>[6x]MTRRYLKYYIFVTLLFFVQVINNVLCAPDNKQEQGKYLNRTINILNAGKNIAKSYGHNKLKPIHILSALAKSDYGSTLFKENNVNAANLKEYIDIALEQTRAGAPLDNKSKIVNSAEVKETLALAEAAANKYKSPKVDVEHLLSGLSNDELVNEIFNEVYLTDEAIKAILKRKFEKTKKDKDGKTGTLYIEQFGSNMNEKVRNGKLQGIYGRDEEIRAIIESLLRYNKNSPVLVGNPGTGKTTIVEGLVYRIEKGDVPKELQGYTVISLNFRKFTSGTSYRGEFETRMKNIIKELKNKKNKIILFVDEIHLLLGAGKAEGGTDAANLLKPVLSKGEIKLIGATTIAEYRKFIESCSAFERRFEKILVEPPSVDMTVKILRSLKSKYENFYGINITDKALVAAAKISDRFIKDRYLPDKAIDLLNKACSFLQVQLSGKPRIIDVTERDIERLSYEISTLEKDVDKVSKKKYNKLI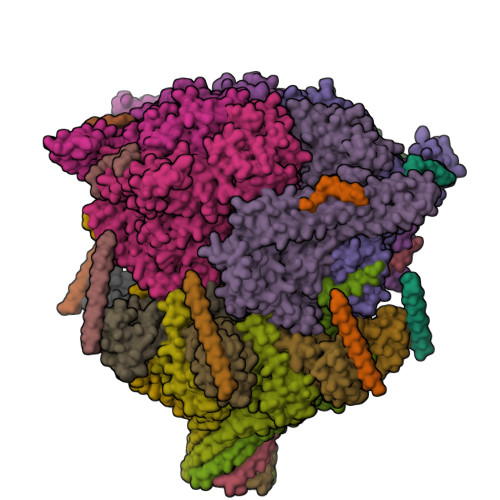KEFEEKKEQLKKYYEEYVITGERLKRKKEIEKKLNDLKELTQNYVYSNKEPPIELQNSLKEAQQKYLELYKETVAYVEAKTHNAMNVDAVYQEHVSYIYLRDSGMPLGSLSFESSKGALKLYNSLSKSIIGNEDIIKSLSDAVVKAATGMKDPEKPIGTFLFLGPTGVGKTELAKTLAIELFNSKDNLIRVNMSEFTEAHSVSKITGSPPGYVGFSDSGQLTEAVREKPHSVVLFDELEKAHADVFKVLLQILGDGYINDNHRRNIDFSNTIIIMTSNLGAELFKKKLFFDADNSGTPEYKRVMEDVRLSLIKKCKKVFKPEFVNRIDKIGVFEPLNKKNLHKIVALRFKKLEKRLEEKNIQVSVSEKAIDYIIDQSYDPELGARPTLIFIESVIMTKFAIMYLKKELVDDMDVFVDYNSKAKNLVINLSKT;>MKVSYIFSFFLLFFVYKNTNTVVCDNGYGDLAATSALTTVIKDPISLTIKDIYEHGVKNPFTKIIHKLKKFIRYRKVLRWSRMWWVLLVREIVGDNTIEKKTEKALREIWDQCTIAVYNNTLNAVESKPLLFLHGILNECRNNFATKLRQDPSLIVAKIDQIIKSQIYRFWVSEPYLKIGRSHTLYTHITPDAVPQLPKECTLKHLSSYMEEKLKSMESKKNIESGKYEFDVDSSETDSTKDDGKPDDDDDDDDNFDDDDNFDDDTVEEEDASGDLFKNEKKDENKE[7x];>MRIIILALLIVCTIINYYCAVQNNGNKSLNVMPTCSMPGNDSDSNDNETGDVDNDKNNELGNANDNNEMNNENAESKNMQGENSNNQEQLNENVHANDDAMYEGTPSSDNPPQENVDANNNEQEYGPPQEEPVSENNVENVEVATDDSGNDNINNNDNFNNNDNYNDNDNFNEEPPSDDGNKNEDELTEGNQSDDKPMNEEEATINEMGKITNPFEDMLKGKVDDMDIGKMMNKDNLQSFLSSLTGNKDGSGKNPLSDMMNIFGVPQTGKEGAEGGVNKENQMKQINELKDKLETMLKGAGVNVDKIKDSIKNNDLLKNKQLLKEAISKLTLDPSMMNMLNNKDGANGKPFDINPDSMMKMFNALSNENGNLDDLKMKPTDGSFDSFNDGVDNNLVPSNPKGQNNNEEDDEEGGDDDDYDDKSFVVNSKYADNSFEDKFNTFDEKDDDVKYELFGENEEAEELNNNTTTASSKGDANNSVNTQEGEGEEESFSANEENINNNNNHNNKNYNNYNTSQQEEDDNSFNENDEPLISSSQFDNNKKNKMSVSTHNKKSKNLMDSLDLESTNYGSNSSSSMSNNYNSKNKNSKKNNKKKSSQKDYIRTDGKVSFDMATLQKTIKNFGGADNEIVQNILKKYVTIDNDDDNDADEDEDEDDDDDDDLDEDEFSVKDIKKLIEEGILDYEDLTENELRKLAKPDDNFYELSPYASDEKDLSLNETSGLTNEQLKNFLGQNGTYHMSYDSKSIDYAKQKKSEKKEDQQEDDDGFYDAYKQIKNSYDGIPNNFNHEAPQLIGNNYVFTSIYDTKENLIKFLKKNSEYDLYDDDDKEGGNFKSPLYDKYGGKLQKFKRQRAFNILKQWRAKEKKLKEKKKKEEMEENKEFDFSKNYNFSSKNDGGVTMFSKDQLEDMVKNFGGKPSAHVTDSFSRKENPFVPTNTKNNSNDDDDMDNGYVTFDGKNKVSENDDDEKGNNNDDENDNDDSNDEEELDEEEDDN[7x]> MDREAFVQTLTACRLCPRLVAWREEVVGRKRAFRGEPYWARPVPGFGDPEARILLFGLAPGAHGSNRTGRPFTGDASGAFLYPLLHEAGLSSKPESLPGDDLRLYGVYLTAAVRCAPPKNKPTPEELRACARWTEVELGLLPEVRVYVALGRIALEALLAHFGLRKSAHPFRHGAHYPLPGGRHLLASYHVSR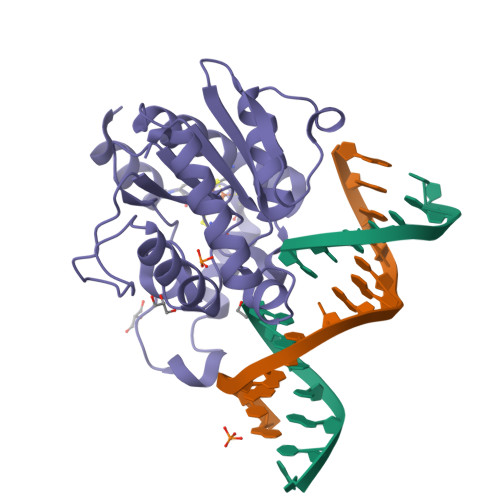QNTQTGRLTREMFLEVLMEAKRLAGL>[2x]QEAEYTLRLHHFFPASAPVHQEYFLPWKEAIEKESDGRLAVELYPSMQLGGTPPSLYDQAKDGQVDIIWTVLGYNSGRFPRAEVFDLPFLPTSGAATSQAAHEYAMTHMQDELEGVYPIAVHTHSPGALHTKETRIEALEDIEGLKMRGPSRLVNRYLAKLGAEPIGMPVAQALEALSRGVLDGTVIPFEAITAMGLADITTEHTIFSGDRALYTTMMIVAMDQDKYDALPEDLQPIIDAHAGGREA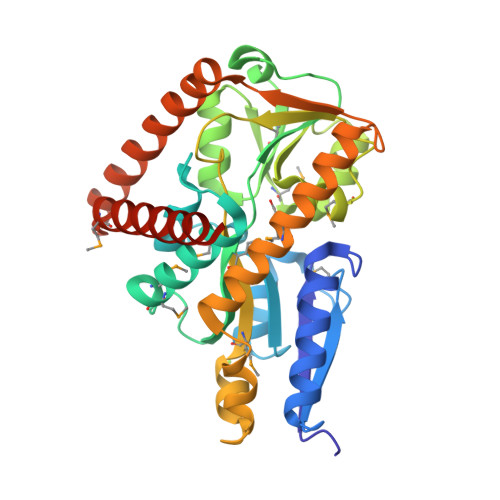YRIGQIMDQADHRQILAIQSGEQPGTITRLGSEETARWQAVGQEVVDEWIAEAEEKGLDGQMLYDDATRLVERYTRAAALEHHHHHH>RNPVLAGLSVEEIREAVSGEYLIEPREEKMVEQVVIGAMSPQSALRYLREARNAALVTGGDRSDLLLTALEMPNVRCLILTGNLEPVQLVLTKAEERGVPVILTGHDTLTAVSR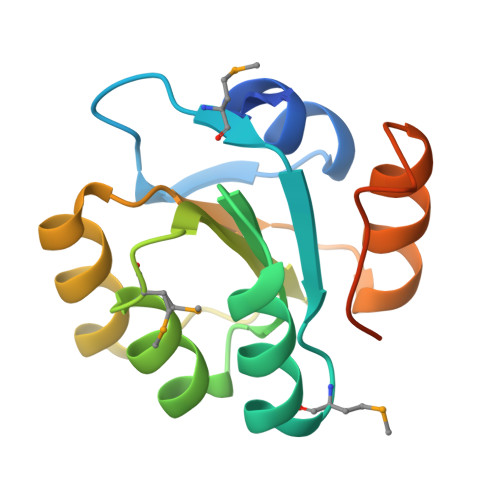LESVFGRTRIRGEPKVGIMRELFES[2x]>[4x]HHHHHHENLYFQGMEKVTVTLDERSYPIN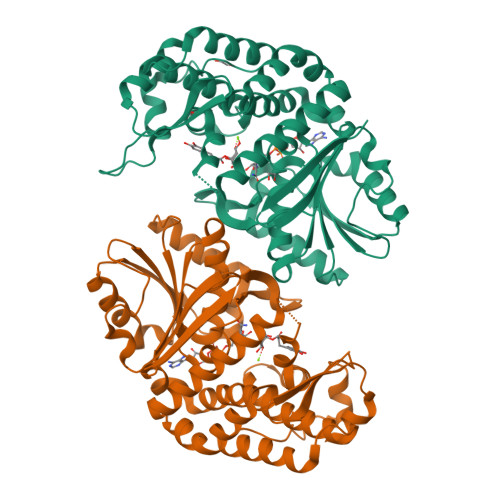IAPSLYQQQDAFWPLTAGQRAMIVTNETLAPLYLHKIQTVLEVSGVKVDSIILPDGEQYKSLFIMNDVFTALLEKHHNRDTTLIALGGGVIGDLTGFAAASYQRGVRFIQVPTTLLSQVDSSVGGKTAVNHPLGKNMIGAFYQPASVVIDLDCLKTLPKRELSSGLAEVIKYGIILDGEFFSWLEENIDALMALDNQAMAYCIRRCCELKAQVVAADEKETSGLRALLNLGHTFGHAIEAEMGYGVWLHGEAVAAGMVMAAKTAELIGQFTPEQTDRVIALLKRAELPVTGPAKMQPDDYLPHMMRDKKVMGGKLHLILPTTIGHSEMRSDVDASTVTAAISACIP> YVATRDNCCILDERFGSYCPTTCGIADFLNNYQTSVDKDLRTLEGILYQVENKTSEARELVKAIQISYNPDQPSKPNNIESATKNSKSMMEEIMKYETLISTHESTIRFLQEIYNSNSQKIVNLRDKVVQLEANCQEPCQDTVKIHDVTGRDCQDVANKGAKESGLYFIRPLKAKQQFLVYCEIDGSGNGWTVFQKRLDGSLDFKKNWIQYKEGFGHLSPTGNTEFWLGNEKIH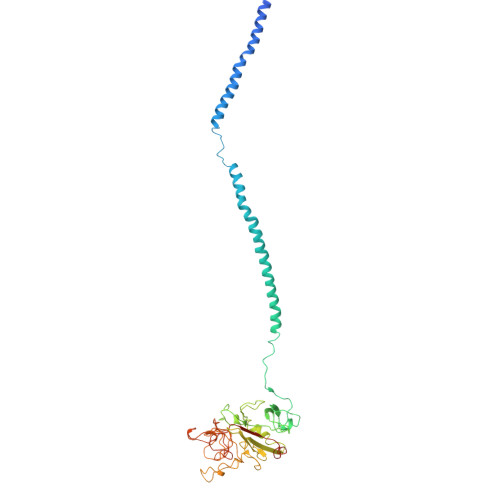LISTQSTIPYVLRIQLEDWNGRTSTADYASFKVTGENDKYRLTYAYFIGGDAGDAFDGYDFGDDSSDKFFTSHNGMQFSTWDSDNDKYDGNCAEQDGSGWWMNKCHAGHLNGVYYQGGTYSKTSTPNGYDNGIIWATWKSRWYSMKKTTMKIIPLNRLAIGEGQQHQLGGAKQAGDV> MAQQSTKNETALLVAKSAKSALQDFNHDYSKSWTFGDKWDNSNTMFETFVNKYLFPKINETLLIDIALGNRFNWLAKEQDFIGQYSEEYVIMDTVPINMDLSKNEELMLKRNYPRMATKLYGNGIVKKQKFTLNNNDTRFNFQTLADATNYALGVYKKKISDINVLEEKEMRAMLVDYSLNQLSETNVRKATSKEDLASKVFEAILNLQNNSAKYNEVHRASGG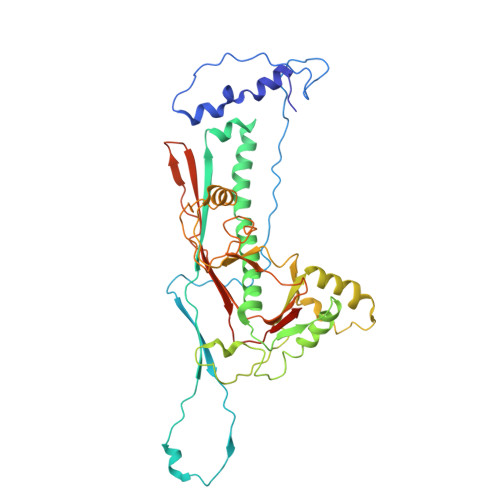AIGQYTTVSKLKDIVILTTDSLKSYLLDTKIANTFQIAGIDFTDHVISFDDLGGVFKVTKEFKLQNQDSIDFLRAYGDYQSQLGDTIPVGAVFTYDVSKLKEFTGNVEEIKPKSDLYAFILDINSIKYKRYTKGMLKPPFHNPEFDEVTHWIHYYSFKAISPFFNKILITDQDVNPKPEEELQE> GSAMGNYMGNPWTEYMAKYDIEEVHGSGIRVDLGEDAEVAGTQYRLPSGKCPVFGKGIIIENSNTTFLTPVATGNQYLKDGGFAFPPTEPLMSPMTLDEMRHFYKDNKYVKNLDELTLCSRHAGNMIPDNDKNSNYKYPAVYDDKDKKCHILYIAAQENNGPRYCNKDESKRNSMFCFRPAKDISFQNYTYLSKNVVDNWEKVCPRKNLQNAKFGLWVDGNCEDIPHVNEFPAIDLFECNKLVFELSASDQPKQYEQHLTDYEKIKEGFKNKNASMIK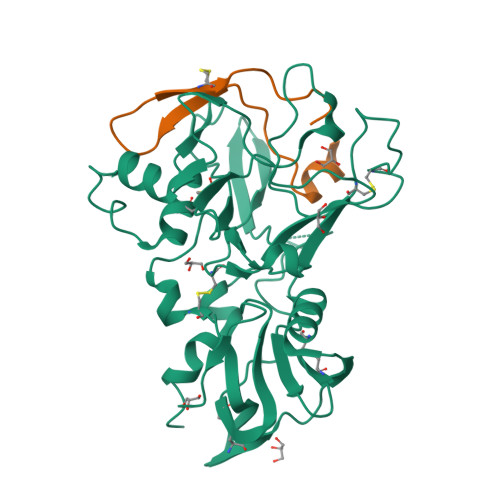SAFLPTGAFKADRYKSHGKGYNWGNYNTETQKCEIFNVKPTCLINNSSYIATTALSHPIEVEAAALVPR;> DITQQAKDIGAGPVASCFTTRMSPPQQICLNSVVNTALS> MSELEKAMVALIDVFHQYSGREGDKHKLKKSELKELINNELSHFLEEIKEQEVVDKVMETLDNDGDGECDFQEFMAFVAMV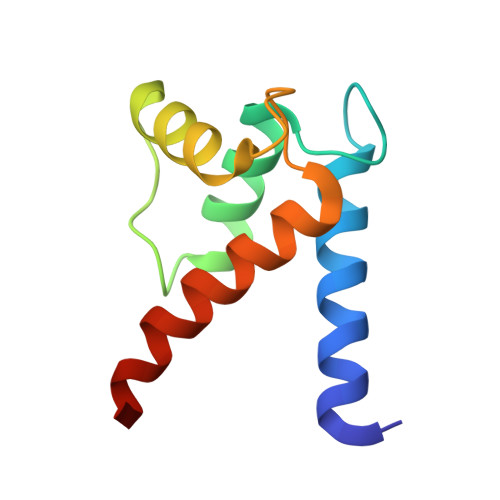TTACHEFFEHE> MSGSLSRGNGGKKVLNKNQLLKRNRIRNARSIRAEAVAASSTKTGTPSDLSESGSKLNVDQFISSRQFEVKQLQLAMHNSKAASSTRIFQALPRKLRRRTASHNVRRIPKRMRNRALREMRKSDQQDVLKGSSASSRKAHGLNAKQLYKARMSIKLLRLASKSTSMKLSMPPEVTSSNCHVRQKIKTLKRMIKESSTANPNIKLLNNRMGSYDCTGVNELAPIPKGRVKYTKRQKHFAWLPTHIWNAKRSHMMKRWGYQMVWAPTQKCFKLTHRLGGDTCSSDGALCMDSSYI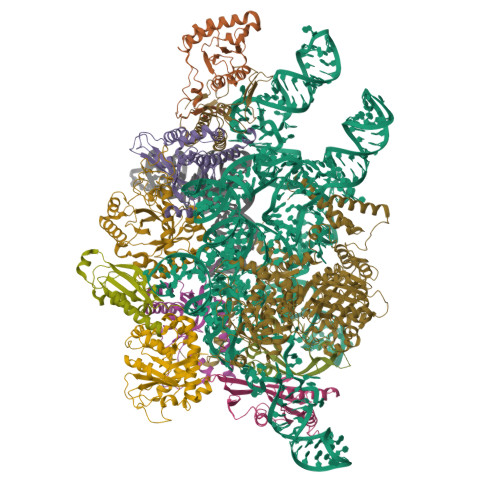GTIIVKDKSNDSEGDFLKSIIGKLTAERANLRKYREGQVLFQGLIYSFNEENGEDSTKPLGPCDVFWVQKDTAIIRLHPSIYTQVFNILLQHKEKLTVQDCRYSLASVTLKGAKALESLASCLRSTEYSKSFEQFKMVSMITDHNALPQRCTFAFEAIDPRHLAAPKKLNDSQRKTVNSDDILSLHENYPQDEINAVFNELCDPESRTQSYNNQNTLKEISARRYKLLTATPNSINKTTVPFKESDDPSIPLVIIRRLKTRDWIVVLPWFWLLPLWHLLNRIPRMYHIGLRQFQQIQYENKQLYFPDDYPFTQLGYIENSFYKKEASKTKWDRKPMGKRINFEKIKDIHNTKLPAYSGEIGDFFSSDWRFLQILRNGIDYLQRNDKTLELMDSKKTGQFNAQGVRDINCVNDVLEFCKDYEAKTKAMSLSIEENIPVALCKNRKCQFRTPDSISVNSSSFSLTFFPRCIIAVSCTLLERGHPKDNARIYQVPEKDLEHWLQLAKGVYRPNGRKDHDLKIPLPEVHDLIGFITSGTYHLNCGNGMGIGFIDHHAAIRQPTRYVLIRNVGTNTYRLGEWSKISV;> MSGSLKSLDKKIAKRRQVYKPVLDNPFTNEAHMWPRVHDQPLIWQLLQSSIINKLIHIQSKENYPWELYTDFNEIVQYLSGAHGNSDPVCLFVCNKDPDVPLVLLQQIPLLCYMAPMTVKLVQLPKSAMDTFKSVSKYGMLLLRCDDRVDKKFVSQIQKNVDLLQFPWLNAIKYRPTSVKLLKTTVPIVSKKRQK;> MDRTQTFIKDCLFTKCLEDPEKPFNENRFQDTLLLLPTDGGLTSRLQRQQRKSKLNLDNLQKVSQLESADKQLEKRDYQRINKNSKIALREYINNCKKNTKKCLKLAYENKITDKEDLLHYIEEKHPTIYESLPQYVDFVPMYKELWINYIKELLNITKNLKTFNGSLALLKLSMADYNGALLRVTKSKNKTLIGLQGIVIWDSQKFFIMIVKGNIIDEIKCIPKKGTVFQFEIPISDDDDSALRYSILGDRFKYRSVDRAGRKFKSRRCDDMLYYIQN;> MVRLKSRYILFEIIFPPTDTNVEESVSKADILLSHHRASPADVSIKSILQEIRRSLSLNLGDYGSAKCNSLLQLKYFSNKTSTGIIRCHREDCDLVIMALMLMSKIGDVDGLIVNPVKVSGTIKKIEQFAMRRNSKILNIIKCSQSSHLSDNDFIINDFKKIGRENENENEDD;> MINGVYYNEISRDLDISSSTQCLRFLKETVIPSLANNGNNSTSIQYHGISKNDNIKKSVNKLDKQINMADRSLGLQQVVCIFSYGPHIQKMLSILEIFKKGYIKNNKKIYQWNKLTSFDIKREGRNELQEERLKVPILVTLVSDSEIIDLNLHSFTKQ;> MALKKNTHNKSTKRVTKHPSLKTLTHKQIHTTIFVKSTTPYVSALKRINKFLDSVHKQGSSYVAVLGMGKAVEKTLALGCHFQDQKNKKIEVYTKTIEVLDEVITEGQADIDMESDVEDDDKETQLKKRAVSGVELRIYV;> MGKKTFREWQYFKLSITSFDQDVDDAHAIDQMTWRQWLNNALKRSYGIFGEGVEYSFLHVDDKLAYIRVNHADKDTFSSSISTYISTDELVGSPLTVSILQESSSLRLLEVTDDDRLWLKKVMEEEEQDCKCI;>MLVDLNVPWPQNSYADKVTSQAVNNLIKTLSTLHMLGYTHIAINFTVNHSEKFPNDVKLLNPIDIKRRFGELMDRTGLKLYSRITLIIDDPSKGQSLSKISQAFDIVAALPISEKGLTLSTTNLDIDLLTFQYGSRLPTFLKHKSICSCVNRGVKLEIVYGYALRDVQARRQFVSNVRSVIRSSRSRGIVIGSGAMSPLECRNILGVTSLIKNLGLPSDRCSKAMGDLASLVLLNGRLRNKSHKQTIVTGGGSGNGDDVVNDVQGIDDVQTIKVVKRSMDAEQLGHASKRHKP[2x];> MGKKAHGGKMKPEIDENGTLLVPPPRTIANQDHFHRLNYLYQISAYQTRARQKARTDAHTPLARNYIKSMDLISKKTKTSLLPTIKRTICKKCHRLLWTPKKLEITSDGALSVMCGCGTVKRFNIGADPNYRTYSEREGNLLNS> RGNNGNMTFNYYANTYQNSVDFSTSSSASGAGPGNSRGGLAGLLT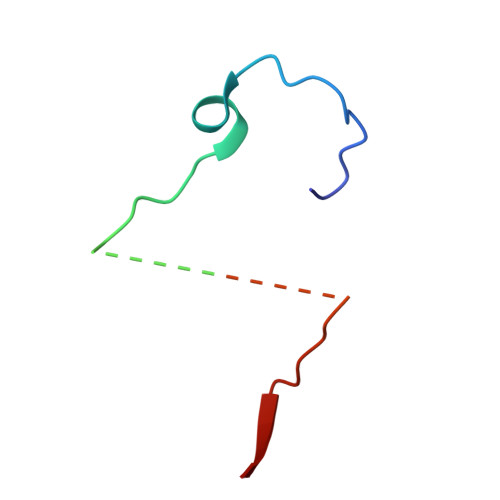NFSGILNPLGYLK>[20x]EEDL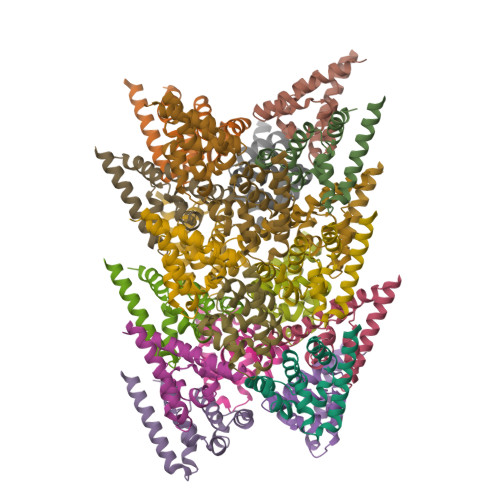TEVKKDALENLRVYLCEKIIAERHFDHLRAKKILSREDTEEISCQTSSRKRAGKLLDYLQENPKGLDTLVESIRREKTQNFLIQKITDEVLKLRNIKLEHLK estrone 3-sulfate | C18 H22 O5 S | 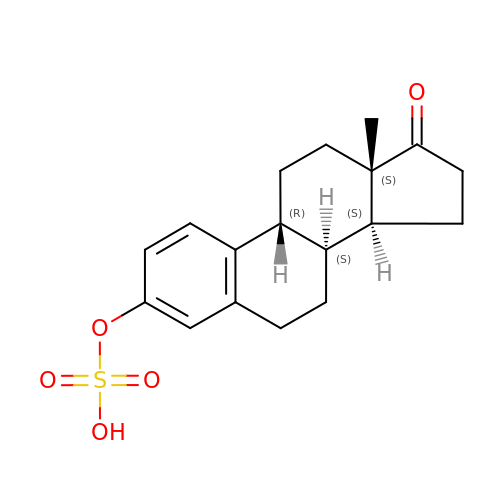JKKFKPJIXZFSSB-OVWQWFNUSA-N(2S)-AMINO[(5S)-3-CHLORO-4,5-DIHYDROISOXAZOL-5-YL]ACETIC ACID | C5 H7 Cl N2 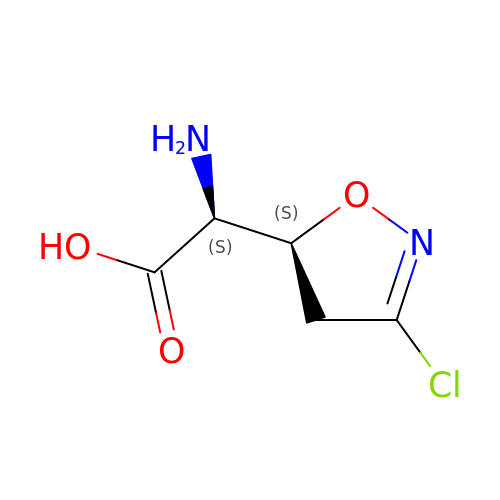O3 | QAWIHIJWNYOLBE-OKKQSCSOSA-N>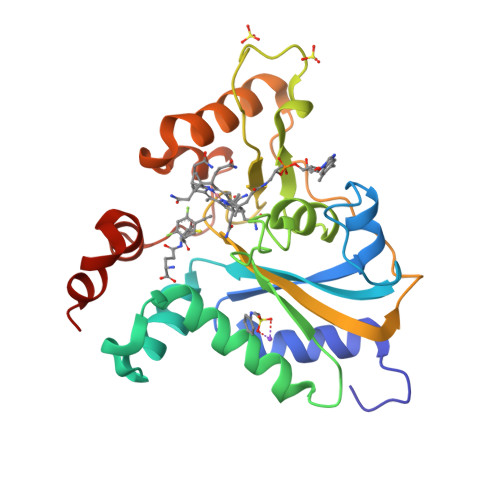 SNAMEPKVAELKQKIEDTLCPFGFEVYPFQVAWYNELLPPAFHLPLPGPTLAFLVLSTPAMFDRALKPFLQSCHLRMLTDPVDQCVAYHLGRVRESLPELQIEIIADYEVHPNRRPKILAQTAAHVAGAAYYYQRQDVEADPWGNQRISGVCIHPRFGGWFAIRGVVLLPGIEVPDLPPRKPHDCVPTRADRIALLEGFNFHWRDWTYRDAVTPQERYSEEQKAYFSTPPAQRLALLGLAQ>[2x]MLIFDDKNYKVDTCNIDGISIKFRSFKEILYCEKPVDSIQKMNIFVPEVYYEGNTINGYSLHTAPIFMPNTVGGYMPGPADEPGKDFKGRINSIFRALKHGYIVVSAGVRGRTSGVKTNEFFVGSKAGEISNENGKMVGRAPALVVDMKAAIRYLRYNKGRIPGNTECIVTNGTSAGGALSAIIGASGNSEDYNPYLKEIGAADERDDIFAASCYCPIHNLENADAAYEWQFCGYNDYHRIKHVRSESGVKNIQIDGILTEKQIKISEELKRLFPKYLNSLKLKDSSNNELLLDENGEGSFKEYIKKLVINSAQKELDLCSTYKIIDNAAVCGSKIDEQEYLSIEDEKVVDINWDGFIKKITRMKVAPAFDALDLKSPENEEFGTEAIKAKHFTAYSQEHSEVEGTLADPKIIKLLNPIEYINNSDTAKYWRVRHGAFDRDISLAMPSILSLTLENNGYVVDFSLPWGIPHSGDYDLDDLFAWIDEIYTK

The biological degradation of water-soluble gallotannins, such as tannic acid, is initiated by tannase enzymes (EC 3.1.1.20), which are esterases able to liberate gallic acid from aromatic-sugar complexes. Here, for the first time, we biochemically and structurally characterize three tannases from a single organism, the anaerobic bacterium Clostridium butyricum, which inhabits both soil and gut environments. In each structure, the catalytic triad and gallate-binding regions in the core domain were found in very similar positions in the active site compared with other bacterial tannases, suggesting a similar mechanism of action among these enzymes, though large inserts in each enzyme showcase overall structural diversity. Furthermore, we solved the structure of one of the enzymes (CbTan2) using X-ray crystallography and have modeled the structures of the other two enzymes (CbTan1 and 3) for comparative analyses.

The crystal structure of CbTan2 was solved to 2.22 Å resolution and conformed to the expected α/β hydrolase fold, while also possessing a cap covering the active site as seen in the two previously solved bacterial tannase structures. The apo structure of CbTan2 contained two protein molecules in the asymmetric unit. A single peak was observed using size-exclusion chromatography, and comparison to a calibration curve revealed that the protein was monomeric in solution (calculated MW ≈ 51 kDa versus expected MW ≈ 55 kDa), which suggests that the dimer observed in the structure is crystallographic and not of biological relevance. The overall structure adopted the α/β hydrolase fold (6 α-helices and 8 β-sheets) with multiple inserts that formed additional 12 helices and five β-sheets, which is similar to the additional inserts observed in other crystallized bacterial tannases. A hairpin-style cap region over the active site was identified in CbTan2, formed by residues 237 to 258, and comprised of two antiparallel β-strands connected by a turn in a hairpin (β8 & 9), similar to the cap identified in TanLp. It appears that the cap of CbTan2 adopts a similar shape and may also be flexible to help accommodate very large substrates, such as environmentally derived tannins that are more complex than the model substrates used here. The catalytic triad of CbTan2 could be identified as Ser175, Asp439, and His471, which is consistent with the enzyme being a subtype B tannase, i.e., possessing a catalytic Asp residue. The catalytic serine residue is found in the sequence motif G-X-S-X-G (Gly173-Thr174-Ser175-Ala176-Gly177), which is conserved across bacterial tannases. In CbTan2, the oxyanion hole appears to be formed by the backbone nitrogen atoms of Gly74 and Ala176. A disulfide bridge was observed between C320 and C332 in both chains; however, residues 321 to 331 (α7 to η4) could not be modeled in chain B due to lack of electron density in this region.4-[(E)-({1-carboxy-2-[(3R)-3-hydroxy-2-oxo-2,3-dihydro-1H-indol-3-yl]ethan-1-id-1-yl}iminio)methyl]-2-methyl-5-[(phosphonooxy)methyl]pyridin-1-ium-3-olate 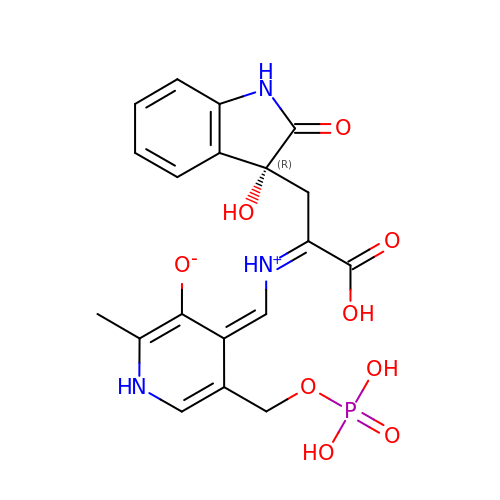| C19 H20 N3 O9 P | KVWUPOTUZSGNFK-JWWNMXMMSA-N The X-ray crystal structure of the capsule polymerase Bcs3 reveals a multi-enzyme machine adopting a basket-like shape that creates a protected environment for the synthesis of the complex Hib polymer. Supported by biochemical studies and comprehensive 2D nuclear magnetic resonance, our data explain how the ribofuranosyltransferase CriT, the phosphatase CrpP, the ribitol-phosphate transferase CroT and a polymer-binding domain function as a unique multi-enzyme assembly. The Bcs3 protomers build into a physiological and functional head-to-tail dimer, which is assembled primarily by interactions between CriT from one protomer and CroT’/CrpP’ from the neighbor protomer, with an overall basket-like shape. CroT transfers ribitol-phosphate from CDP-ribitol, generating a phosphodiester bond with the 3-OH of the nonreducing end ribose of the Hib polymer.

To study the location of Hib capsule polymer in Bcs3, crystals were soaked with oligomer fractions having a narrowed degree of polymerization (DP). A structure was solved by molecular replacement methods (3.6 Å maximum resolution) showing Bcs3 in complex with two complete repeating units (DP2) of the Hib capsule polymer and an additional nonreducing end phosphate coming from a third repeating unit. Bcs3-DP2 crystallized in the P 1 21 1 space group, with four molecules in the asymmetric unit. The overall architecture between Bcs3-CMP and Bcs3-DP2 is essentially preserved. However, we observed more flexibility for the CroT domain in Bcs3-DP2 than for the CroT domain in Bcs3-CMP. DP2 is clearly visible in the electron density maps and is present in all four Bcs3 molecules bound to an SH3b domain (residues 1,037–1,115), with the nonreducing end facing toward the active centers in the main groove. SH3b domains are the prokaryotic counterparts of the well-characterized SH3 domain family. The SH3b domain in Bcs3-DP2 revealed a completely conserved fold—a compact β-barrel, formed by two anti-parallel, three-stranded β-sheets. Notably, Bcs32–1093 and Bcs32–1068, in which the SH3b domain is disrupted, were completely inactive, strongly supporting the mechanistic role of the SH3b domain for Hib capsule polymer recognition.

>[4x]GPVDKTWLFGSYAWQGNPKALFLYMLVNCKETHECWWVADNEESMKSIKKSTGLKNITFTDSEKAKELFPHADVYVTENFRESYPVYMNENIKVFNTWHGVGLKHIELALGMNSVLAESIVRKYVRNYDIYKNNVLFLTTSQAMEDHFLEDMAISKELIIRGKYPRNAVYGPNGIHTYDINTLLPKNKSQYSQTILFCPTYRIGAIQGVLNSLLPDFAKLEEVCRHKNQLFIVKVHPFMKKDNYFAEMSEKYKDSEYILFWNDDYDIYEAFNSIDLAIIDYSSIFYDLLDAGVEKFIRYVPDLDEYQNDLELIGDYADLTEGRIVKSFQQLLNCLDNANIKIISTKRKQYLMDYFFGFKKENKSMESLIADVDNCQLQPKSLKELHTFDIFDTLIRRSTLRPFSIFDYVRDKAKASGIKFPLALTENWINVRNRAEHDVRDIMRKTTFERQSDKIEITLDDIYTRLQKNLLLTDEQTDFLKQAEIEAEIAHVEPIQKRINYLFSLKAKGHDVAMASDMYLPEDVIYKMLDRADTRLREIPLYLSSTIGYQKSTGKLYQHIFFDLDYQYSRWTHYGDNKHADGSVPRRLGIQTAVHDIDDFIPFENAMVNAMDNYNRYPAYQLATKMHRYRTQLVQENGFGNTLFETKYYNYAYVGASFVPYINWAIKDAIKRGYETIYFISRDGHFLKQIADKIIEIRGYNVKTKYIYGSRKAWRLPSFITKVDDETFWQFGNFVGMDSFEDLVKASYLSESELLSLFPEFESLRHAKHLRGEIAENIRKIFKNSPAYHEKVLAIAAEKRKMVRQYIQQEINPKEKFAFVEFWGRGYTQDTFGRLLNDAFGKEVKNPFYYVRSFTDDMGTSVRHNFILAPQNFSFFEPIFAQTPYDSIPDYYEEKGRIEPIINHRDRSVSDLISEGLLKFTEDYLALNTQDEDYFDAALSQFNYQYQLNTPNDQFICNVFSELKDNISSFGVEKPYAPALTLKQLESITSKQELDKLTQSIPISLSKSDVKVIDYYNKIQKNYNLPAYNSTPMRKAYAVNPLEQYVWSTQVPFRVLSLKQNSFYLDVSFAETTKRKDIFLKELNEIDVIAVDWLKGGVPRLLTEHGYITAHKDWVKKSFNDDKTNNIEEPKVKNKEKSKVLEVNTTVTNNNKQAIGKLDNNIDKSLEHHHHHH>[2x]MSELFSERIPPQSIEAEQAVLGAVFLDPAALVPASEILIPEDFYRAAHQKIFHAMLRVADRGEPVDLVTVTAELAASEQLEEIGGVSYLSELADAVPTAANVEYYARIVEEK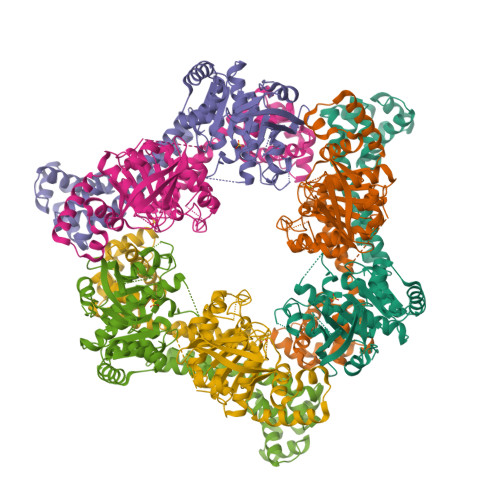SVLRRLIRTATSIAQDGYTREDEIDVLLDEADRKIMEVSQRKHSGAFKNIKDILVQTYDNIEMLHNRDGEITGIPTGFTELDRMTSGFQRSDLIIVAARPSVGKTAFALNIAQNVATKTNENVAIFSLEMSAQQLVMRMLCAEGNINAQNLRTGKLTPEDWGKLTMAMGSLSNAGIYIDDTPSIRVSDIRAKCRRLKQESGLGMIVIDYLQLIQGSGRSKENRQQEVSEISRSLKALARELEVPVIALSQLSRSVEQRQDKRPMMSDIRESGSIEQDADIVAFLYRDDYYNKDSENKNIIEIIIAKQRNGPVGTVQLAFIKEYNKFVNLERRFDEAQIPPGA> DPMKNTCKLLVVADHRFYRYMGRGEESTTTNYLIELIDRVDDIYRNTAWDNAGFKGYGIQIEQIRILKSPQEVKPGEKHYNMAKSYPNEEKDAWDVKMLLEQFSFDIAEEASKVCLAHLFTY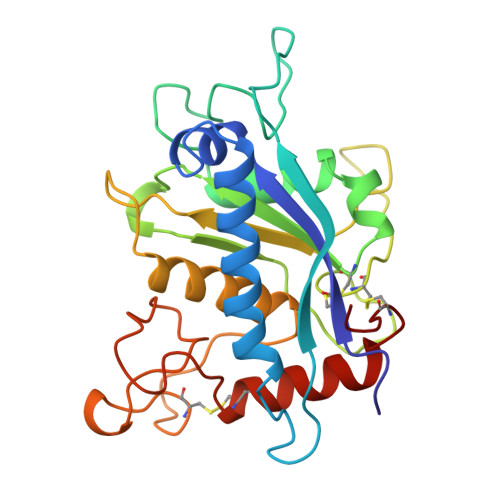QDFDMGTLGLAYVGSPRANSHGGVCPKAYYSPVGKKNIYLNSGLTSTKNYGKTILTKEADLVTTHELGHNFGAEHDPDGKAECAPNEDQGGKYVMYPIAVSGDHENNKMFSQCSKQSIYKTIESKAQECFQERS>MSKAGASLATCYGPVSADVMAKAENIRLLILDVDGVLSDGLIYMGNNGEELKAFNVRDGYGIRCALTSDIEVAIITGRKAKLVEDRCATLGITHLYQGQSNKLIAFSDLLEKLAIAPENVAYVGDDLIDWPVMEKVGLSVA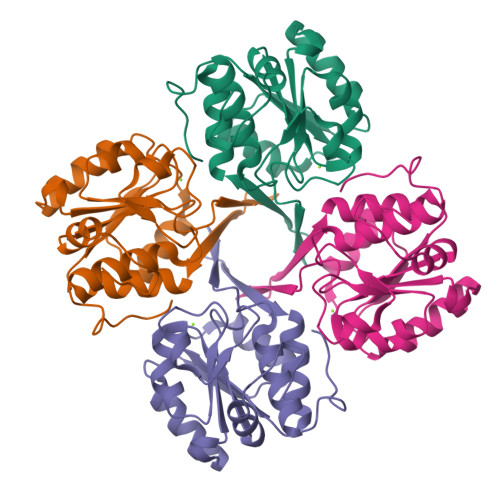VADAHPLLIPRADYVTRIAGGRGAVREVCDLLLLAQGKLDEAKGQSI[8x]>MASIKKVYRGMKNGAETINDDLEAINSELTSGGNVVHKTGDETIAGKKTFTGNVEVNGSLTLPTKSWSGELGGGIILSLRKKGTTVEYSIGGEISSSILANSNLVNRSVPNEFCPRNRCSLVGHMVG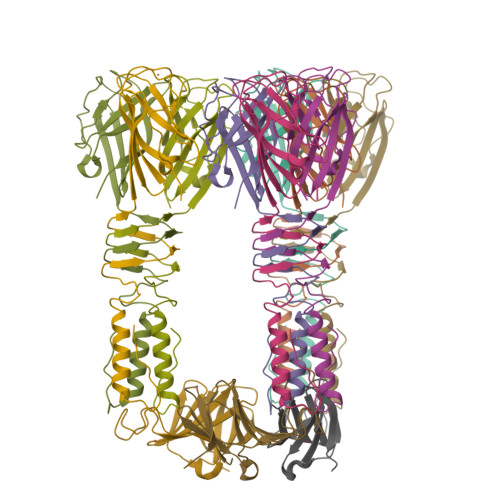GWNAFHIDIPSSGVCQWFGPTASSGTPRGTGTYPIDH[18x];>[6x]GFKFVLEHDSEYQPEVKVTSYKNAIGTETDGFDSGPVFGGGTIYNVPVSLSYDRQKVYVEMPKSYTLAGDIILIDDGTLLVIKETQVLCFKMSDAKITKGYVFVA> MTVFRQENVDDYYDTGEELGSGVFAVVKKCREKSTGLQYAAKFIKKRRTKSSRRGVSREDIEREVSILKEIQHPNVITLHEVYENKTDVILILELVAGGELFDFLAEKESLTEEEATEFLKQILNGVYYLHSLQIAHFDLKPENIMLLDRNVPKPRIKIIDFGLAHKIDFGNEFKNIFGTPEFVAPEIVNYEPLGLEADMWSIGVITYILLS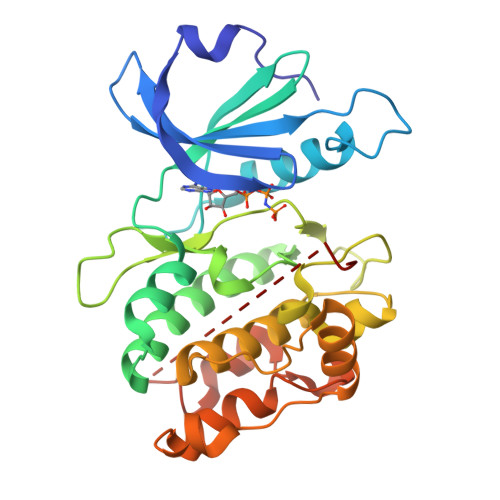GASPFLGDTKQETLANVSAVNYEFEDEYFSNTSALAKDFIRRLLVKDPKKRMTIQDSLQHPWIKPKDTQQALSSAWSHPQFEK Diphosphoinositol phosphates (PP-InsPs) are an evolutionarily ancient group of signalling molecules that are essential to cellular and organismal homeostasis. The PP-InsPs are formed through the enzymatic phosphorylation of myo-inositol hexakisphosphate (InsP6) by inositol hexakisphosphate kinases (IP6Ks) and diphosphoinositol pentakisphosphate kinases (PPIP5Ks). Among the PP-InsPs, 5-diphospho-myo-inositol pentakisphosphate (5-PP-InsP5, also known as “5-InsP7”) is both the most abundant and the most intensively studied member of this signalling family. Metabolically-stable PP-InsP analogues can also be informative for structural analysis of enzyme/substrate crystal complexes.

We then obtained an X-ray structure of 5-PCF2Am-InsP5 (1) in complex with PPIP5K2 kinase domain and the stable ATP analogue AMPPNP. The structure shows that 5-PCF2Am-InsP5 binds to the catalytic site of PPIP5K2 in a similar orientation to 5-PP-InsP5. While crystallography previously showed that 5-PA-InsP5 binds to two sites in PPIP5K2 (the catalytic site and a surface-mounted ligand capture site), electron density for 1 was seen only in the catalytic site. The electron density for 1 clearly shows that the planar amide unit adopts the Z conformation, and with the amide NH antiperiplanar to H-5 of myo-inositol. The carbonyl oxygen of the amide is orientated similarly to one non-bridging oxygen atom of the α-phosphate of bound 5-PP-InsP5. Additionally, one of the fluorine atoms in the CF2 group stretches its position to that of the other non-bridging O-atom of an α-phosphate, which is expected to bring the negative charge distribution in this region closer to that of 5-PP-InsP5 than occurs with the PA analogue. The terminal phosphonate group in bound 1 is held in an extended conformation although its orientation is different to that of the corresponding β-phosphate group in 5-PP-InsP5 bound to PPIP5K2. Note also that the 5-diphosphate in 5-PP-InsP5 participates in complexing a hydrated Mg2+ ion, a property that is mimicked in the complex of 5-PCP-InsP5 with PPIP5K2.7 This Mg2+ ion is not present in the complex with 1. Compound 1 inhibited 1,5-[PP]2-InsP4 metabolism by PPIP5K2 with an IC50 of 375 nM. In addition, the rigidity of the amide unit in 1 means that the PCF2Am unit contains fewer rotatable bonds than the equivalent PP, PA or PCP structures.

> GSFTERQIVVGICSMAKKSKSKPMKEILERISLFKYITVVVFEEEVILNEPVENWPLCDCLISFHSKGFPLDKAVAYAKLRNPFVINDLNMQYLIQDRREVYSILQAEGILLPRYAILNRDPNNPKECNLIEGEDHVEVNGEVFQKPFVEKPVSAEDHNVYIYYPTSAGGGSQRLFRKIGSRSSVYSPESNVRKTGSYIYEEFMPTDGTDVKVYTVGPDYAHAEARKSPALDGKVERDSEGKEVRYPVILNAREKLIAWKVCLAFKQTVCGFDLLRANGQSYVCDVNGFSFVKNSMKYYDDCAKILGNIVMRELAPQFHIPWSIPLEAED>[9x]MPLTNLTPTELLANKAVDYLANSFLVETPMLGLLANRVINQKQKAIEWGAKVAQGVVGGRTRTGALANDTQGTIKGASLSVPDYYIKHQFDVGKDEIVNSDATGKISAVRDPVGTAIADAFDVLSKKINSVLYTASGVADATNYGIFGLDAAAGTTV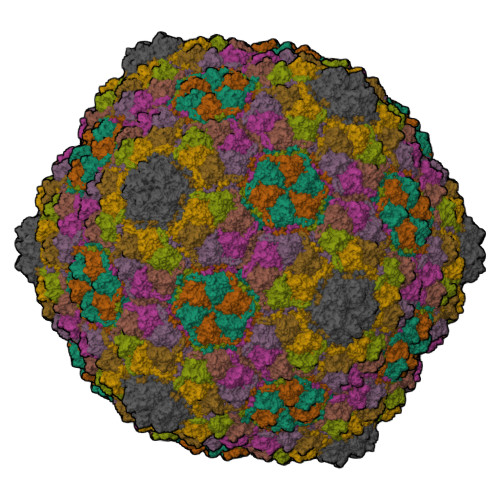ANSATGTYAGISKVTFPRWRSIIQGGAVPGTNEALTIARMTAMLRARRTAGVTYKGNQNQRLVILTSDNIENDVLRPLYGTVVDNQNVDFTRLDKDLLPYVNYMVKGIPVVSDIDCPANKMYLLNLDKLAIYSFDQSDADQSNGKITYIPLRYVDETGDTPSESTLWVRLADVSDEHPDLLKFELSVALQLVAFDLIDSISVIRDITQ>[2x]MPELPPPHVVREAEKARADLQRQSRELAPPPFALLELIMGVMVTRAVHVAAELKVAEALAEGPLSADELAGRVGADADALGRVLRLLASNGVFATRPDGAFELTPMADALRADHPMSMRGIALLMGHPIHWEDWSGFPETVVTGEPALPKLRGMHAFEFLTKNAEYGQVFFQGMGSMSASETEPILAAYDFSQFGTVVDFCGGQGALLAGILGAAPGCEGVLFDPRVEENGAAEFLAAQGVADRTKRVAG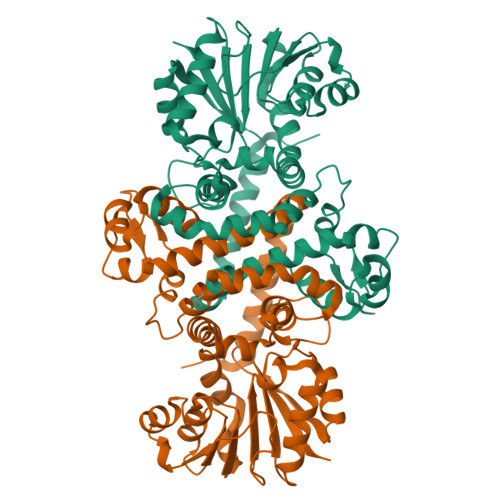DLFDVPPGGADAYVLKHIVHDWPEEQALRILRNVRAAIKPGGKLLIAEMVIPEQGDQPHSGKLVDLWLMLLVGGRERTPGQYADLLARAGFRLERVVETAAAISLVEAVPV>[2x]GHMTLGEELSRRRRLLNSITELK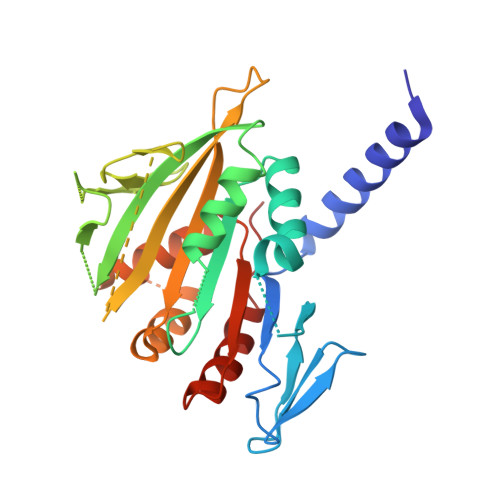GCARLFANIIEDEISEKLIVNYSDESIEDMKNHKTYKFTKLIQNFSHQNKDLFKEDLHVYIDFCLKRRENFNLFSVGSSNIPNTFEKLLAFFKNNYFDKFVITLQYVMLSDNADSQDLLSNNKDGGKDVEIKLKIEESTISLGSTLITLDEITDKLQIKKKYSQLNHQNGIGLSKFQFFCLQDIEPIPIDFYFIEIYQPSIYPILKRSTGTESNLNSPLEIVLKKIFHDTKSAFVFQIDHSAEVYDILKLSSHLSFIRNPKGK> MAQASSTPAVSPRPRPRYREERTLVRKLLPRPGQSKQEFRENVKKLRKAFLQFNADVSGVCQWAIQFRPRYGKPAEPTETFWKFFLEPETSLPPNDSRSPEFRRLQAFEAAAGINGAAALDDPAFTNELRDSILAVASRPKTKEAQRLFSRLKDYQPAHRMILAKVAAEWIESRYRRAHQNWERNYEEWKKEK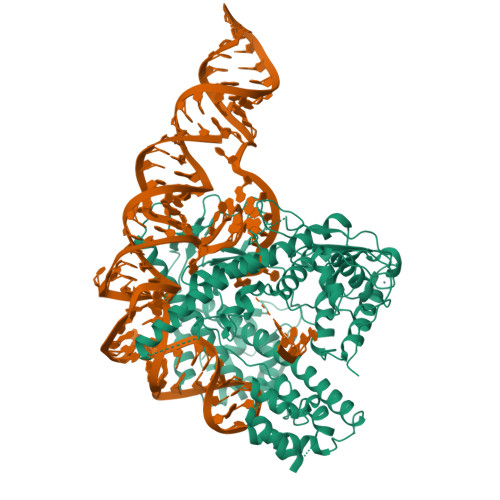QEWEQNHPELTPEIREAFNQIFQQLEVKEKRVRICPAARLLQNKDNCQYAGKNKHSVLCNQFNEFKKNHLQGKAIKFFYKDAEKYLRCGLQSLKPNVQGPFREDWNKYLRYMNLKEETLRGKNGGRLPHCKNLGQECEFNPHTALCKQYQQQLSSRPDLVQHDELYRKWRREYWREPRKPVFRYPSVKRHSIAKIFGENYFQADFKNSVVGLRLDSMPAGQYLEFAFAPWPRNYRPQPGETEISSVHLHFVGTRPRIGFRFRVPHKRSRFDCTQEELDELRSRTFPRKAQDQKFLEAARKRLLETFPGNAEQELRLLAVDLGTDSARAAFFIGKTFQQAFPLKIVKIEKLYEQWPNQKQAGDRRDASSKQPRPGLSRDHVGRHLQKMRAQASEIAQKRQELTGTPAPETTTDQAAKKATLQPFDLRGLTVHTARMIRDWARLNARQIIQLAEENQVDLIVLESLRGFRPPGYENLDQEKKRRVAFFAHGRIRRKVTEKAVERGMRVVTVPYLASSKVCAECRKKQKDNKQWEKNKKRGLFKCEGCGSQAQVDENAARVLGRVFWGEIELPTAIP> MEIPVIEPLFTKVTEDIPGAEGPVFDKNGDFYIVAPEVEVNGKPAGEILRIDLKTGKKTVICKPEVNGYGGIPAGCQCDRDANQLFVADMRLGLLVVQTDGTFEEIAKKDSEGRRMQGCDDCAFDYEGNLWITAPAGEVAPADYTRSMQEKFGSIYC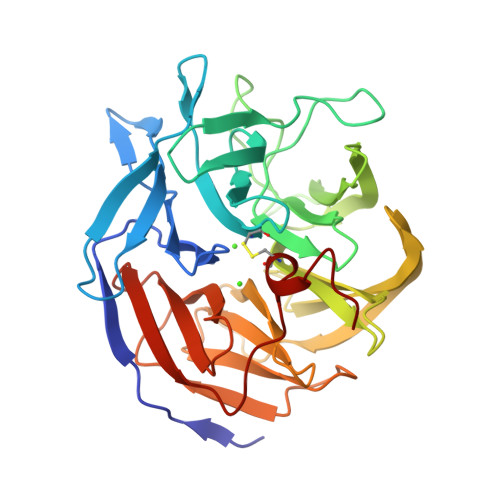FTTDGQMIQVDTAFQFPNGIAVRHMNDGRPYQLIVAETPTKKLWSYDIKGPAKIENKKVWGHIPGTHEGGANGMDFDEDNNLLVANWGSSHIEVFGPDGGQPKMRIRCPFEKPSNLHFKPQTKTIFVTEHENNAVWKFEWQRNGKKQYCETLKFGIF[(2R,3S,4R,5R)-5-(6-amino-2-fluoro-9H-purin-9-yl)-3,4-dihydroxytetrahydrofuran-2-yl]methyl [(2R,3S,4S)-3,4-dihydroxytetrahydrofuran-2-yl]methyl dihydrogen diphosphate | C15 H22 F N5 O13 P2 | 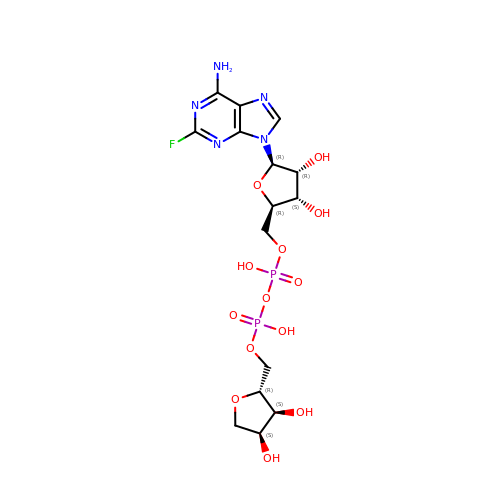INVLSELIWGCOEO-ZVIMGNLFSA-N> PPVIAPRPEHTKSIYT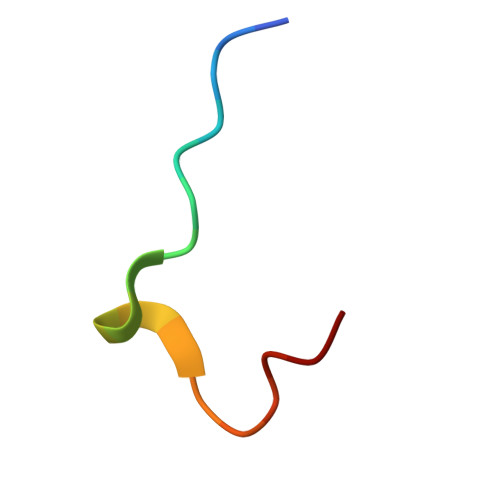RS> GPLGSWSWESYLEEQKAITAPVSLFQDSQAVTHNKNGFKLGMKLEGIDPQHPSMYFILTVAEVCGYRLRLHFDGYSECHDFWVNAN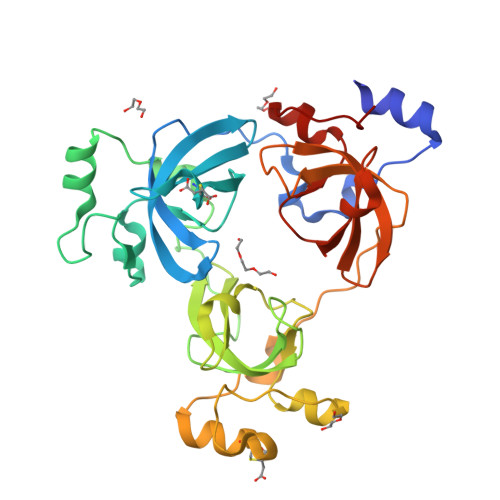SPDIHPAGWFEKTGHKLQPPKGYKEEEFSWSQYLRSTRAQAAPKHLFVSQSHSPPPLGFQVGMKLEAVDRMAPSLVCVASVTDVVDSRFLVHFDNWDDTYDYWCDPSSPYIHPVGWCQKQGKPLTPPQDYPDPDNFCWEKYLEETGASAVPTWAFKVRPPHSFLVNMKLEAVDRRNPALIRVASVEDVEDHRIKIHFDGWSHGYDFWIDADHPDIHPAGWCSKTGHPLQPPLG> MEQETLEQVHLTEDGGVVKTILRKGEGGEENAPKKGNEVTVHYVGKLESSGKVFDSSRERNVPFKFHLGQGEVIKGWDICVASMTKNEKCSVR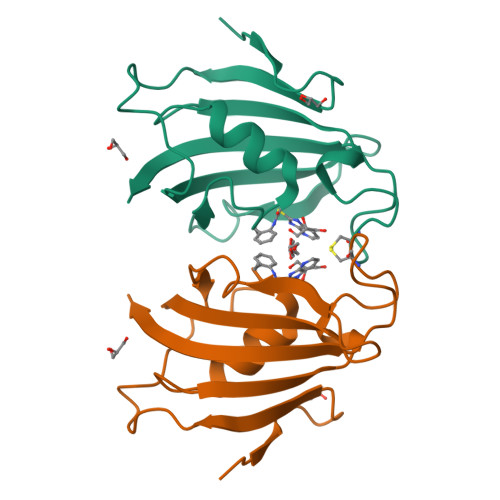LDSKYGYGEEGCGESIPGNSVLIFEIELISFRE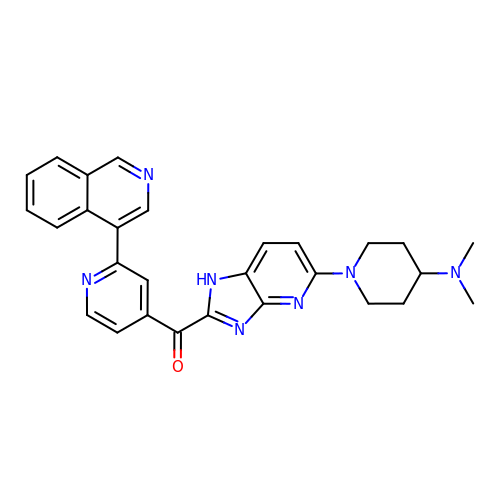{5-[4-(dimethylamino)piperidin-1-yl]-1H-imidazo[4,5-b]pyridin-2-yl}[2-(isoquinolin-4-yl)pyridin-4-yl]methanone | C28 H27 N7 O | VSHURSPEQITHNX-UHFFFAOYSA-N In mammals, the most abundant and best-studied NDPKs are NME1 and NME2 (hereafter abbreviated NME1/2), which are closely related isoforms (88% sequence identity) with similar functional attributes and localization in the cytosol and nucleus. NME1/2 are hexameric enzymes that catalyze the reaction XTP + YDP ⇆ XDP + YTP by first transferring the γ-phosphoryl group from XTP (usually ATP) to residue His118, and then from the phosphohistidine to YDP, where Y is any of the four common (deoxy)nucleosides. Briefly, each NME1 subunit within the D3-symmetric hexamer comprises an antiparallel four-stranded β sheet flanked on either side by a layer of helices. In this study, we showed that NME1 binds AcCoA and CoA with similar affinity via a binding mode distinct from that of canonical ADP and ATP substrates and critically dependent on the CoA 3′ phosphate group.

Efforts to cocrystallize murine NME1 with the ligands led to high-resolution (1.96 and 2.2 Å, respectively) crystal structures of NME1 bound to SucCoA and ADP, and a somewhat lower (2.6 Å)–resolution structure bound to CoA. CoA and SucCoA bind to this site via their common nucleotide moiety, the only part of these ligands specifically recognized by NME1. Second, the high resolution of our NME1/SucCoA crystal structure revealed several water molecules structurally conserved across hexamer subunits that play an important role in compensating for the shift of CoA nucleotide atoms relative to their counterparts in ADP. Important water molecules are numbered 1 to 6. Three of these are conserved between the ADP- and SucCoA-bound structures. The CoA 3′ phosphate group forms direct H bonds with Lys12, Tyr52, Asn115, and His118 as well as water-mediated H bonds with Arg88, Arg105, and the Gly119 backbone. Compared to ADP, the α and β phosphates of CoA are displaced upward and are solvent accessible, pointing out of the pocket to direct the CoA pantetheine end away from the protein surface. Consequently, the acyl-bearing end of CoA remains solvent accessible when bound to NME1 and potentially free to interact with other protein partners, consistent with our findings that NME1 binds similarly to acylated and non-acylated CoA. Incubating NME1 with either AcCoA or SucCoA yielded similar spectra, revealing that NME1 does not strongly discriminate between these ligands and CoA. The recorded profiles revealed that the melting temperature of NME1 (Tm = 60°C) was enhanced similarly by each of the tested ligands (ΔTm ≈ 3.7°C), confirming that AcCoA and SucCoA bind NME1 with similar affinity to CoA.

>[12x]GAMAMANSERTFIAIKPDGVQRGLVGEIIKRFEQKGFRLVGLKFLQASEDLLKEHYTDLKDRPFFTGLVKYMHSGPVVAMVWEGLNVVKTGRVMLGETNPADSKPGTIRGDFCIQVGRNIIHGSDSVKSAEKEISLWFQPEELVEYKSCAQNWIYE>MHHHHHHTSKIEQPRWASKDSAAGAASTPDEKIVLEFMDALTSNDAAKLIEYFAEDTMFQAMPLPPAYGRDAVEQTLAGLFTVMSIDAVETFHIGSSNGLVYTERVDVLRALPTGKSYNLSILGVFQLTEGKITGWRDYFDLREFEEAVDLPLRG[2x]

We report an in silico strategy for the biocatalytic synthesis of chiral N- and O-heterocycles via Baldwin cyclization modes of hydroxy- and amino-substituted epoxides and oxetanes using the limonene epoxide hydrolase from Rhodococcus erythropolis. We turned to cofactor-independent limonene epoxide hydrolases (LEHs) that normally catalyze direct hydrolysis of epoxides by positioning and activating water at the active site. On the basis of the well-documented mechanism of ReLEH, a water molecular is positioned by H-bonds to N55 and Y53 while D132 abstracts a proton from the water, enabling a smooth nucleophilic attack on one of the substrate’s epoxide carbon center. We have rationally engineered the epoxide hydrolase ReLEH with construction of a general platform for Baldwin cyclization reactivity of hydroxy- and amino-epoxides and oxetanes.

To further elucidate the mechanism, crystallographic experiments were performed. We obtained the complex crystals of SZ611-substrate 59 and SZ611-product 46 using the soaking methods as described in Material and Methods. SZ611 assembles into a homodimer structure with four α-helices and five-strand β-sheets in each monomer, forming a cavity that serves as a deep substrate-binding pocket, in which a substituent of substrate 59 or of product 46 can occur without steric repulsion. The electron density map of such ligands and surrounding key residues were defined with good quality. A major portion of substrate 59 was clearly defined in the electron density map, apart from a minor portion of the phenyl group. The N-atom of substrate 59 is hydrogen-bonded to D132, which commonly functioned as a proton receptor for the deprotonation of an amine group, or for deprotonation of water molecules in WT LEH and other LEH mutants. Product 46 shares a similar conformation with substrate 59 considering the hydrogen-bonding networks of amines and hydroxyl groups with D132 and D101, which together predicts a pathway for the LEH-catalyzed selective desymmetrization reactions of oxetanes. In the catalytic reactions, residue D132 acts as a proton acceptor to promote the deprotonation of the amino group. The deprotonated N-atom then nucleophilically attacks the oxetane moiety, resulting in ring opening, followed by the protonation of the O-atom of the oxetane precursor with D101 as the proton donor. For the desymmetric oxetane reactions, we propose a putative catalytic pathway, which mainly includes the following crucial processes: (1) deprotonation of the amine group; (2) nucleophilic attack of carbon atom (C2) of the oxetane; (3) protonation of oxygen atom of oxetane.>[2x]GSAKDPMRVLKYAILGLLRKGELSGYDITSYFKEELGQFWSAKHSQIYPE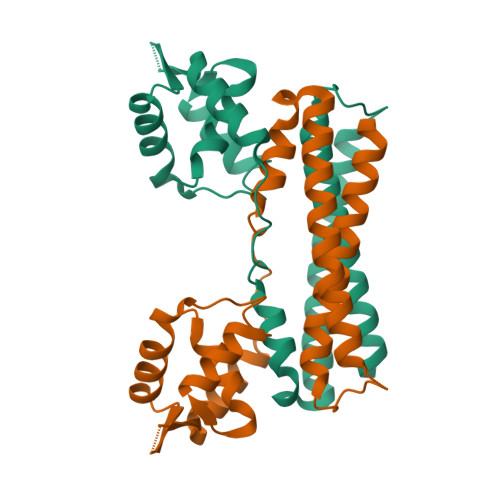LKKLTDEGFITFRTTIQGTKLEKKMYTLTDSGKQELHDWLIRHQPIPETVKDEFMLKAYFISSLSRQEASDLFTDQLLKRKAKLSDLQGSYEKLMASAEPMSFSSPDFGHYLVLTKALEREKNYVSWLESILAMIDED> GPKVPMSQKNGIATLLQAEKEAHEIVSKARKYRQDKLKQAKTDAAKEIDSYKIQKDKELKEFEQKNAGGVGELEKKAEAGVQGELAEIKKIAEKKKDDVVKILIETVIK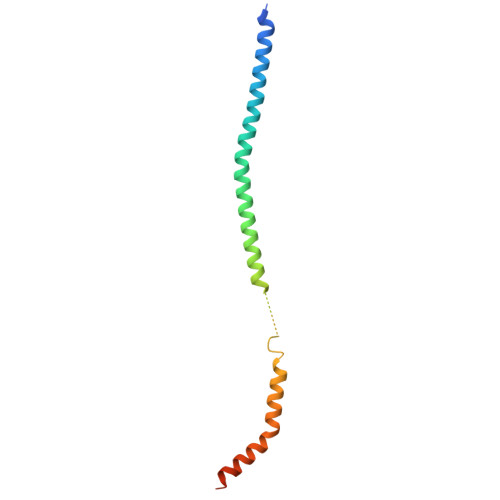PSAEVHINAL>[2x]GSHHHHHHGSHMDEKLLKTIAESKYLVALTGAGVSAESGIPTFRGKDGLWNRYRPEELANPQAFAKDPEKVWKWYAWRMEKVFNAQPNKAHQAFAELERLG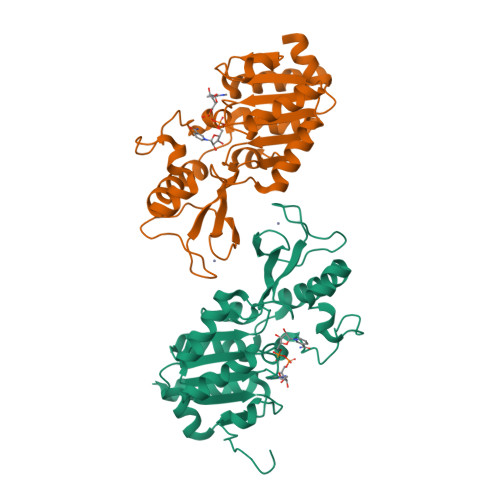VLKCLITQNVDDLHERAGSRNVIHLHGSLRVVRCTSCNNSFEVESAPKIPPLPKCDKCGSLLRPGVVWFGEMLPPDVLDRAMREVERADVIIVAGTSAVVQPAASLPLIVKQRGGAIIEINPDETPLTPIADYSLRGKAGEVMDELVRHVRKALS> MLDAFSRVISNADAKAAYVGGSDLQALRTFISDGNKRLDAVNYIVSNSSCIVSDAISGMICENPGLITPGGNCYTNRRMAACLR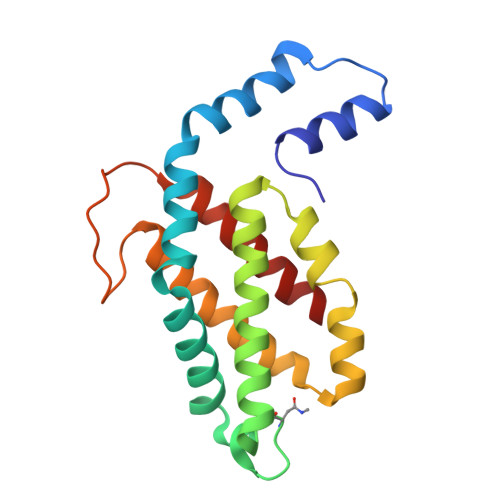DGEIILRYISYALLAGDSSVLEDRCLNGLKETYIALGVPTNSTVRAVSIMKAAVGAFISNTASQRKGEVIEGDCSALAAEIASYCDRISAAVS>[2x]AKMHGAFSTNVVASKELQQPGSARSTRHLEIELPKEASYQEGDHLGVIPRNYEGIVNRVTARFGLDASQQIRLEAEEEKLAHLPLAKTVSVEELLQYVELQDPVTRTQLRAMAAKTVCPPHKVE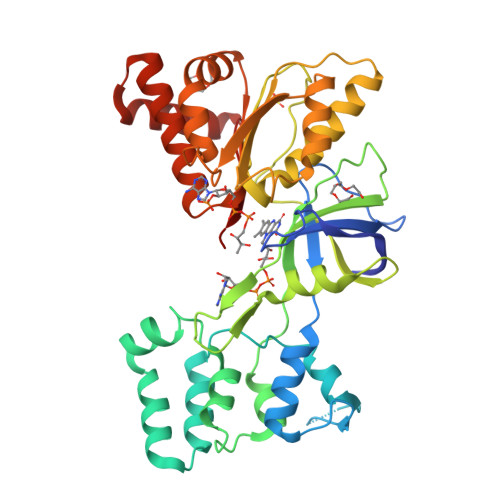LEALLEKQAYKEQVLAKRLTMLELLEKYPACEMKFSEFIALLPSIRPRYYSISSSPRVDEKQASITVSVVSGEAWSGYGEYKGIASNYLAELQEGDTITCFISTPQSEFTLPKDPETPLIMVGPGTGVAPFRGFVQARKQLKEQGQSLGEAHLYFGCRSPHEDYLYQEELENAQSEGIITLHTAFSRMPNQPKTYVQHVMEQDGKKLIELLDQGAHFYICGDGSQMAPAVEATLMKSYADVHQVSEADARLWLQQLEEKGRYAKDVWAG> RSELTIVPDFYPTMVRNFNPYLATNLRTTTDFIYEPLVVFNEMKGNTPVFRLAESYKMADDLMSVTFDIRKGVKWSDGEAFTADDVVYSFGLLKAKPELDQRGINKWVTSVEKVDEYKVRFRLSEANSNVPYEISLIPIVAEHVWKDVKDPTTFTNENPVG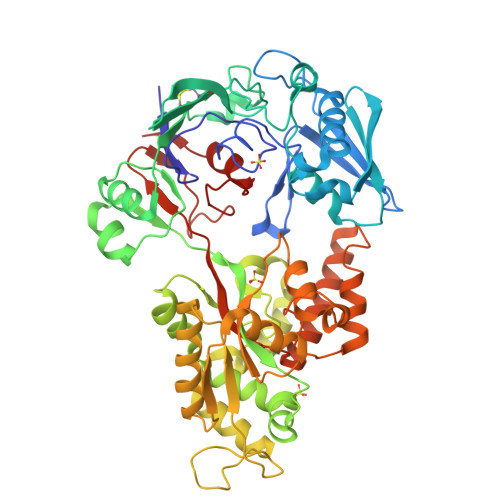TGPFTVIDTFTPQLYIQCRNPNYWDAANLEVDCLRVPQIANNDQLLGKIVNSELDWTSSFVPDIDRTYAAANPNHHYWYPAAGTQAFMVNFKNPDPAKKEALDNVDFRRAFSMALDRQTIIDIAFYGSGTVNDFASGLGYAFEAWSDEATHKKYKGFNTYDVEGSKKLLAKAGFKDVNGDGFVETPSGKSFELLIQSPNGWTDFNNTVQLAVEQLQEVGIKAKARTPEFAVYNQAMLEGTYDVAYTNYFHGADPFTYWNSGYNSALQSGDGMPRFAMHYFTDKKLDGLLDSFYKTADKNEQLAIAHGIQKIIAENQVTIPVMSGAWMYQYNTTRFTGWWSEENPKGRPSVWAGIPERLLHVLDLKPVK>TKVVLGQNQYGKAEVRLVKVTRNTARHEIQDLNVTSQLRGDFEAAHTAGDNAHVVATDTQKNTVYAFARDGFATTEEFLLRLGKHFTEGFDWVTGGRWAAQQFFWDRINDHDHAFSRNKSEVRTAVLEISGSEQAIVAGIEGLTVLKSTGSEFHGFPRDKYTTLQETTDRILATDVSARWRYNTVEVDFDAVYASVRGLLLKAFAETHSLALQQTMYEMG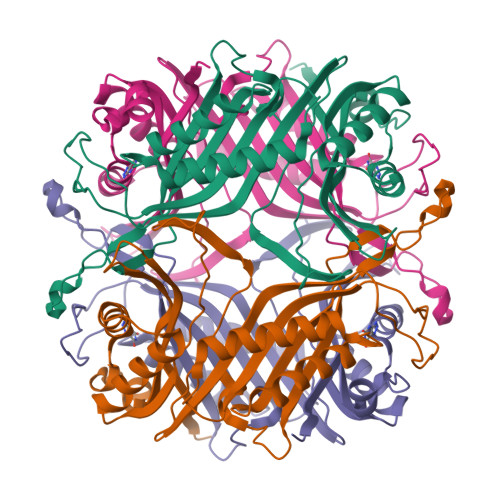RAVIETHPEIDEIKMSLPNKHHFLVDLQPFGQDNPNEVFYAADRPYGLIEATIQREGSRADHPIWSN[8x]> MKSTTPKKITPNVTFCDENAKEPENALDKLFSSEQQASILHVLNTASTKELEAFRLLRGRRSINIVEHRENFGPFQNLESLMNVPLFKYKSTVQVCNSIL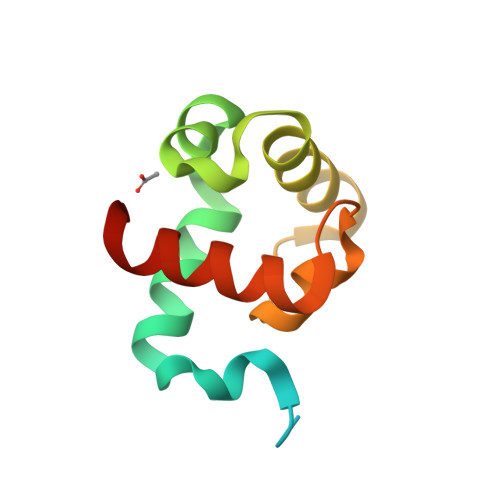HHHHHH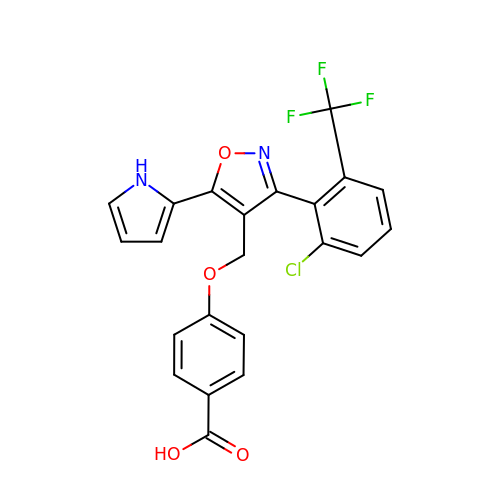4-[[3-[2-chloranyl-6-(trifluoromethyl)phenyl]-5-(1~{H}-pyrrol-2-yl)-1,2-oxazol-4-yl]methoxy]benzoic acid | C22 H14 Cl F3 N2 O4 | RSKUYRRDRPIYIT-UHFFFAOYSA-N>[2x]MMIASSLAVLYGIAIVSSMGVQSARADYADDCTTPDGDQGQCM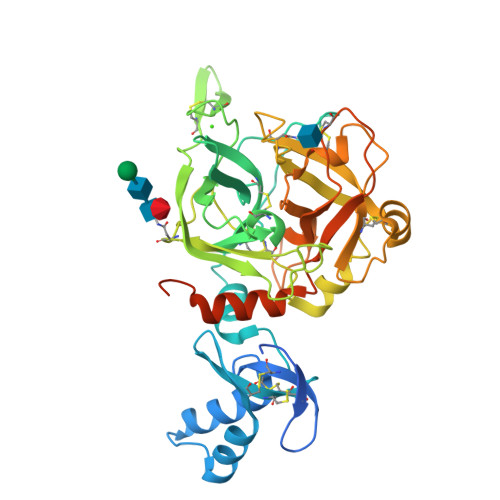PFSSCRTIEERLTEAQKAGQKVPADYASYLQKALCGEFNGVRHFCCPSANIQHNSKVMSLFKDENFDCGNFLSQRVSNGYEVKLSSRPWMALLRYQQFGESRFLCGGAMISERYILTAAHCVHGLQNDLYEIRLGEHRISTEEDCRQQGRKKKCAPPVVNVGIEKHLIHEKYDARHIMHDIALLKLNRSVPFQKHIKPICLPITDELKEKAEQISTYFVTGWGTTENGSSSDVLLQANVPLQPRSACSQAYRRAVPLSQLCVGGGDLQDSCKGDSGGPLQAPAQYLGEYAPKMVEFGIVSQGVVTCGQISLPGLYTNVGEYVQWITDTMASNGLLESRGPFEGKPIPNPLLGLDSTRTGHHHHHH> APMSSAW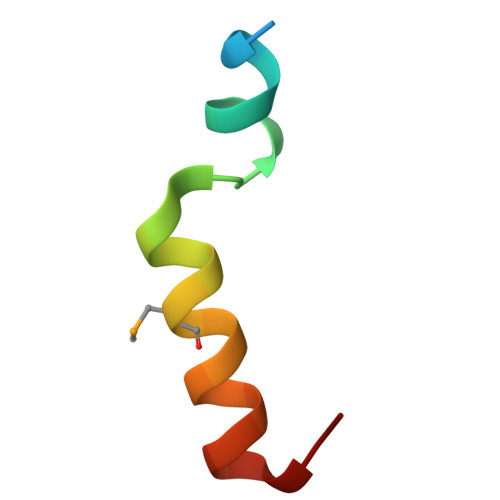KTVACGGTRDQLFMQEKARQLLGRL>GPSPYKEEIEDLKMKLVKIDLEKMKNAKEFEKEISATKATVEYQKEVIRLLRENLRRSQQAQDTSVISEHTDPQPSNKPLTCGGGSGIVQNTKALILKSEHIRLEKEISKLKQQNEQLIKQKNELLSNNQHLS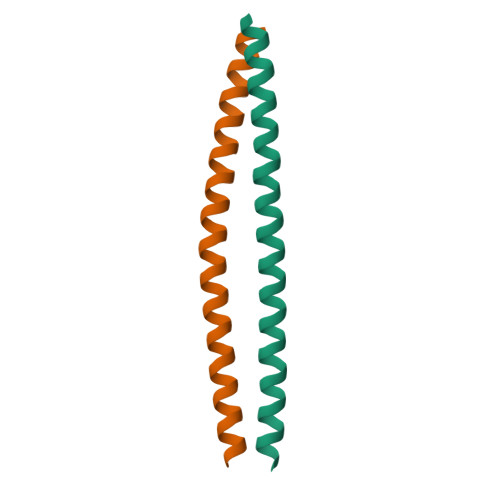NEVKTWKERTLKREAHK[2x]>QKPVVNTAYGRVRGVRRELNNEILGPVVQFLGVPYATPPLGARRFQPPEAPASWPGVRNATTLPPACPQNLHGALPAIMLPVWFTDNLEAAATYVQNQSEDCLYLNLYVPTEDGPLTKKRDEATLNPPDTDIRDSGKKPVMLFLHGGSYM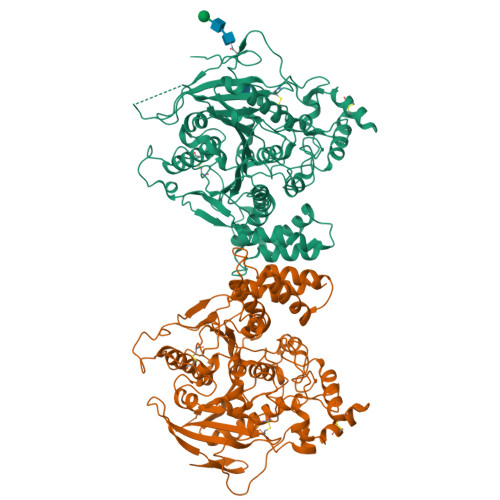EGTGNMFDGSVLAAYGNVIVVTLNYRLGVLGFLSTGDQAAKGNYGLLDQIQALRWLSENIAHFGGDPERITIFGSGAGASCVNLLILSHHSEGLFQKAIAQSGTAISSWSVNYQPLKYTRLLAAKVGCDREDSTEAVECLRRKSSRELVDQDVQPARYHIAFGPVVDGDVVPDDPEILMQQGEFLNYDMLIGVNQGEGLKFVEDSAESEDGVSASAFDFTVSNFVDNLYGYPEGKDVLRETIKFMYTDWADRDNGEMRRKTLLALFTDHQWVAPAVATAKLHADYQSPVYFYTFYHHCQAEGRPEWADAAHGDELPYVFGVPMVGATDLFPCNFSKNDVMLSAVVMTYWTNFAKTGDPNQPVPQDTKFIHTKPNRFEEVVWSKFNSKEKQYLHIGLKPRVRDNYRANKVAFWLELVPHLHNLHHHHHHHH[4x]> MKKSL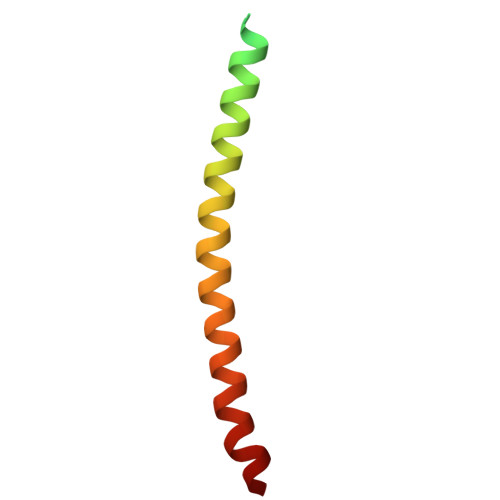VLKASVAVATLVPMLSFAAEGDDPAKAAFNSLQASATEYIGYAWAMVVVIVGATIGIKLFKKFTSKAS>LPIISEGNRNRHRAWALRELQDIKKEIENKAPGSQVWIQTLRLAI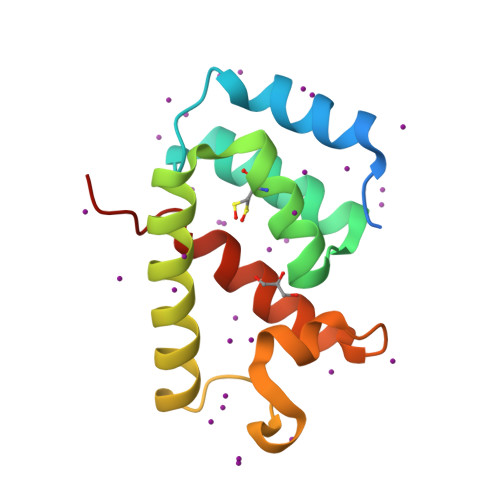LQADPTPADLEQLCQYIASPVDQTAHMTSLTAAIAAAEAANTLQGFNPQNGTLTQQSAQPNAGDLRSQYQNLWLQAWKNLPTRP[2x]> MTDMWDVRITDTSLRDGSHHKRHQFTKDEVGAIVAALDAAGVPVIEVTHGDGLGGSSFNYGFSKTPEQELIKLAAA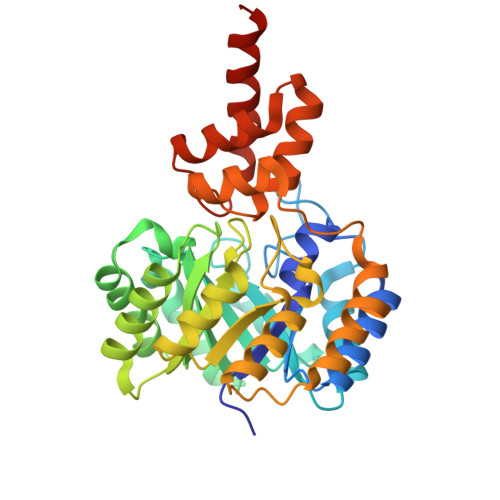TAKEARIAFLMLPGVGTKDDIKEARDNGGSICRIATHCTEADVSIQHFGLARELGLETVGFLMMAHTIAPEKLAAQARIMADAGCQCVYVVDSAGALVLDGVADRVSALVAELGEDAQVGFHGHENLGLGVANSVAAVRAGAKQIDGSCRRFGAGAGNAPVEALIGVFDKIGVKTGIDFFDIADAAEDVVRPAMPAECLLDRNALIMGYSGVYSSFLKHAVRQAERYGVPASALLHRAGQRKLIGGQEDQLIDIALEIKRELDSGAAVTH>[16x]MRGSHHHHHHGSSLFNRGIESPQVLEEHGISVYASIPLSEWQKARDSVKTIKGIKRYKQSQLLAVGNPTDLAIEAIRSLRTSLHFAMMQAQNNVLMMTGVSPSIGMTFVCANLAAVISQTNKRVLLIDCDMRKGYTHELLGTNNVNGLSEILIGQGDITTAAKPTSIAKFDLIPRG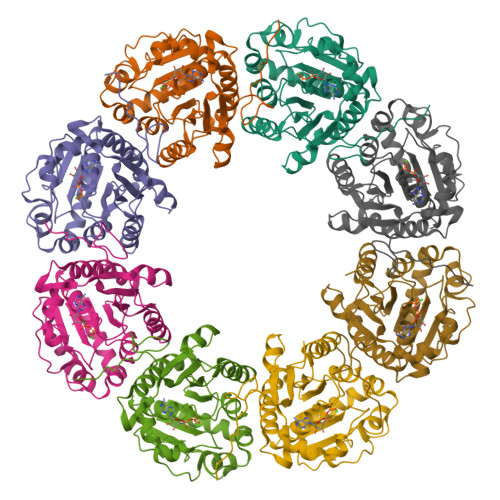QVPPNPSELLMSERFAELVNWASKNYDLVLIDTPPILAVTDAAIVGRHVGTTLMVARYAVNTLKEVETSLSRFEQNGIPVKGVILNSIFRRASAYQDYGYYEYEYKSDAK> WSHPQFEKGGVGKVAQPAAIGGPFQLTDQNGKAVTDKSLKGKPTLIFFGYTHSPDVCPTSLFEISEVLRAMGKDADKVNAIFISVDPERDTPAT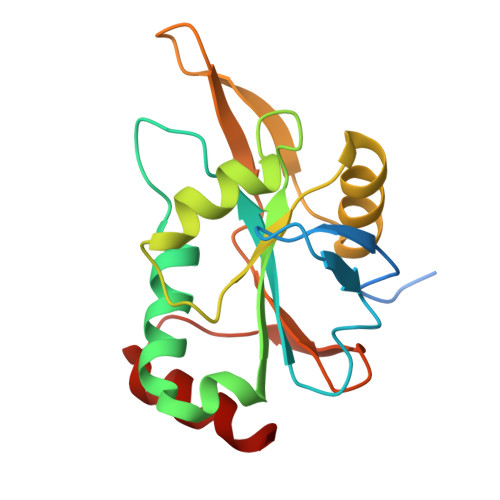MKNYLSSFDPHLEGLSGDPAEIAKVITSYRVYAKKVPTKDGDYTMDHTALIYLMDRDGRFVSPFNLKRTPEEAAADLKRYL(1~{R})-1-methyl-2,3,4,9-tetrahydro-1~{H}-pyrido[3,4-b]indole | C12 H14 N2 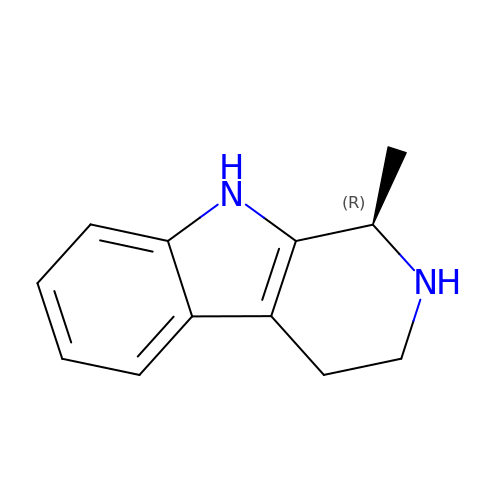| LPIJOZBIVDCQTE-MRVPVSSYSA-N> QELPQMTQQLNSDDMQEQLSATVKFRQILSREHRPPIDVVIQAGVVPRLVEFMRENQPEMLQLEAAWALTNIASGTSAQTKVVVDADAVPLFIQLLYTGSVEVKEQAIWALGNVAGDST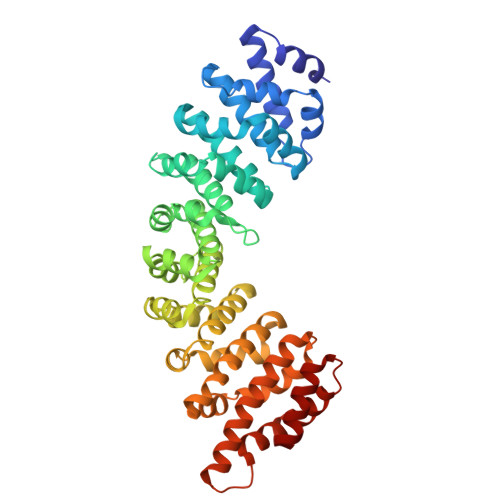DYRDYVLQCNAMEPILGLFNSNKPSLIRTATWTLSNLCRGKKPQPDWSVVSQALPTLAKLIYSMDTETLVDACWAISYLSDGPQEAIQAVIDVRIPKRLVELLSHESTLVQTPALRAVGNIVTGNDLQTQVVINAGVLPALRLLLSSPKENIKKEACWTISNITAGNTEQIQAVIDANLIPPLVKLLEVAEDKTKKEACWAISNASSGGLQRPDIIRYLVSQGCIKPLCDLLEIADNRIIEVTLDALENILKMGEADKEARGLNINENADFIEKAGGMEKIFNCQQNENDKIYEKAYKIIETYF(S)-2-(PHOSPHONOXY)CAPROYL-L-LEUCYL-P-NITROANILIDE | C18 H28 N3 O8 P | 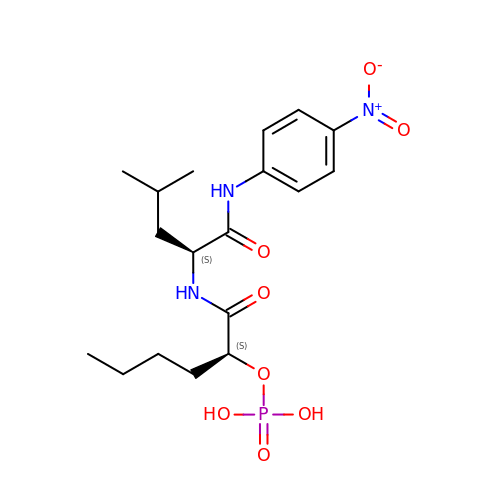HARXAJAHMRMERT-HOTGVXAUSA-N K. pneumoniae use type 1 pili tipped with the two-domain FimH adhesin to cause urinary tract infections (UTIs). FimH interdomain interactions result in a conformational equilibrium between low-affinity and high-affinity forms. The N-terminal mannose-binding lectin domain of FimH (FimHLD) mediates binding to mannose-decorated uroplakins on the surface of bladder epithelial cells and desmoglein-2 in renal epithelial cells, interactions that are essential for disease and can trigger invasion of both UPEC and K. pneumoniae into bladder epithelial cells where they subsequently replicate and form clonal intracellular bacterial communities (IBCs). While the FimHLD binding pocket mediates direct stereospecific recognition of mannose, the interaction of the lectin domain with the pilin domain greatly influences the conformation of the mannose-binding pocket of FimH.

We investigated the structure of the mannose-binding FimH lectin domain truncate (FimHLD) of K. pneumoniae, which is separated from any allosteric effects of the FimH pilin domain. We solved the X-ray crystal structure of TOP52 FimHLD bound to d-mannose to 1.34 Å. A comparison of the structures of UPEC and K. pneumoniae FimHLDs revealed that both FimHs bind d-mannose in a similar fashion with small differences in the orientation of Y48 and Y137, located on binding loops 2 and 3 respectively, which make up a “tyrosine gate” and are involved in binding of mannose ligands. In K. pneumoniae FimHLD, Y48 and Y137 are ~4.2 Å closer to each other compared to UPEC FimHLD. In agreement with the structural similarity, measurements of binding to BSA-mannose by biolayer interferometry showed that K. pneumoniae FimHLD bound to mannose with high affinity (Kd = 7.4 μM) although slightly lower than UPEC FimHLD (Kd = 2.4 μM). We show that the K. pneumoniae FimHLD isolated away from the pilin domain primarily adopts a high-affinity mannose-binding conformation, supporting that interactions between the lectin and pilin domains negatively impact the mannose-binding pocket. Close examination of the crystal structure showed two residue interaction differences at positions 132 and 141 from UPEC at the base of binding loop 3, between the K. pneumoniae residues (H132 and S141) compared to the analogous interaction in UPEC (R132 and D141). We found that only the K. pneumoniae FimHLD H132R/S141D double mutant significantly enhanced binding, reflected by an increase in melting temperature by 2.8 °C for the FimHLD in complex with the high-affinity mannoside Fim1033 (36). These results suggest that the H132/S141 residues in K. pneumoniae FimHLD result in a less flexible binding loop 3 that reduces mannose-binding affinity.

> FACKTATGATIPIGGGSANVYVNLTPAVNVGQNLVVDLSTQIFCHNDYPETITDYVTLQRGSAYGGVLSSFSGTVKYNGTSYPFPTTTETARVIYDSRTDKPWPAVLYLTPVSTAGGVAITAGSLIAVLILHQTNNYNSDSFQFIWNIYANNDVVVPTGGHHHHHH> MDRASELLFYVNGRKVIEKNVDPETMLLPYLRKKLRLTGTKYGCGGGGCGACTVMISRYNPITKRIRHHPANACLIPICSLYGAAVTTVEGIGSTHTRIHPVQERIAKCHGTQCGFCTPGMVMSIYTLLRNHPEPTLDQLTDALGGNLCRCTGYRPIIDACKTFCKTSGCCQSKENGVCCLDQGINGLPEFEEGSKTSPKLFAEEEFLPLDPTQELIFPPELMIMAEKQSQRTRVFGSERMMWFSPVTLKELLEFKFKYPQAPVIMGNTSVGPEVKFKGVFHPVIISPDRIEELSVVNHAYNGLTLGAGLSLAQVKDILADVVQKLPEEKTQMYHALLKHLGTLAGSQIRNMASLGGHIISRHPDSDLNPILAVGNCTLNLLSKEGKRQIPLNEQFLSKCPNADLKPQEILVSVNIPYSRKWEFVSAFRQAQRQENALAIVNSGMRVFFGEGDGIIRELCISYGGVGPATICAKNSCQKLIGRHWNEQMLDIACRLILNEVSLLGSAPGGKVEFKRTLIISFLFKFYLEVSQILKKMDPVHYPSLADKYESALEDLHSKHHCSTLKYQNIGPKQHPEDPIGHPIMHLSGVKHATGEAIYCDDMPLVDQELFLTFVTSSRAHAKIVSIDLSEALSMPGVVDIMTAEHLSDVNSFCFFTEAEKFLATDKVFCVGQLVCAVLADSEVQAKRAAKRVKIVYQDLEPLILTIEESIQHNSSFKPERKLEYGNVDEAFKVVDQILEGEIHMGGQEHFYMETQSMLVVPKGEDQEMDVYVSTQFPKYIQDIVASTLKLPANKVMCHVRRVGGAFGGKVLKTGIIAAVTAFAANKHGRAVRCVLERGEDMLITGGRHPYLGKYKAGFMNDGRILALDMEHYSNAGASLDESLFVIEMGLLKMDNAYKFPNLRCRGWACRTNLPSNTAFRGFGFPQAALITESCITEVAAKCGLSPEKVRIINMYKEIDQTPYKQEINAKNLIQCWRECMAMSSYSLRKVAVEKFNAENYWKKKGLAMVPLKFPVGLGSRAAGQAAALVHIYLDGSVLVTHGGIEMGQGVHTKMIQVVSRELRMPMSNVHLRGTSTETVPNANISGGSVVADLNGLAVKDACQTLLKRLEPIISKNPKGTWKDWAQTAFDESINLSAVGYFRGYESDMNWEKGEGQPFEYFVYGAACSEVEIDCLTGDHKNIRTDIVMDVGCSINPAIDIGQIEGAFIQ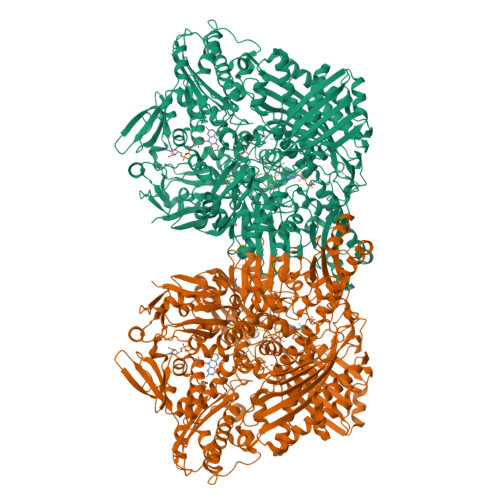GMGLYTIEELNYSPQGILHTRGPDQYKIPAICDMPTELHIALLPPSQNSNTLYSSKGLGESGVFLGCSVFFAIHDAVSAARQERGLHGPLTLNSPLTPEKIRMACEDKFTKMIPRDEPGSYVPWNVPI> MGYYDEDGHYHSFRHGIHKLADKIVHPSGHHHHHHDHIDVDIRETVTGPRPRPGDSGDSYLPNTVTIPCHHIRLGDFLMLQ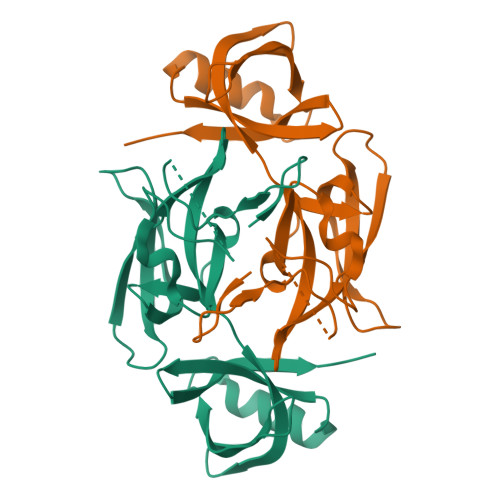GRPCQVIRISTSPATGQYRYLGVDLFTKQLHEESSFISNPAPSVVVQTMLGPVFKQYRVLDMHDGRVVAMTETGDVKQGLAVIDQSNLWSRLHNAFESGRGSVRVLVLNDSGRELAVDMKVIHGSRL>[2x]MSSFDFMSYIITKAELVNKALDSAVPLREPLKIHEAMRYSLLAGGKRVRPVLCIAACELVGGEESTAMPAACAVEMIHTMSLIHDDLP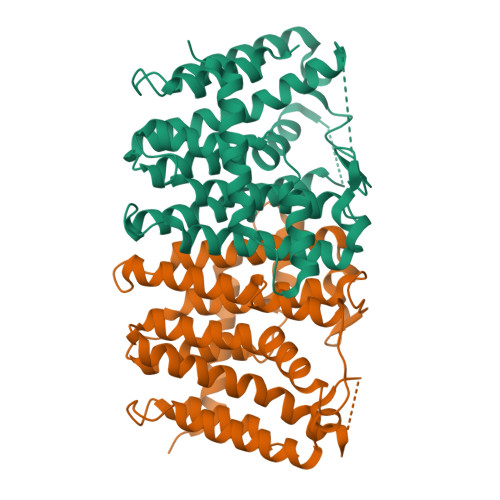CMDNDDLRRGKPTNHKVFGEDVAVLAGDALLSFAFEHLASATSSDVVSPVRVVRAVGELAKAIGTEGLVAGQVVDISSEGLDLNDVGLEHLEFIHLHKTAALLEASAVLGAIVGGGSDDEIERLRKFARCIGLLFQVVDDILDVTKSSKELGKTAGKDLIADKLTYPKIMGLEKSREFAEKLNREARDQLLGFDSDKVAPLLALANYIAYRQNLEHHHHHH>[11x]MSYHKENTPLTAGSQAASSSTASY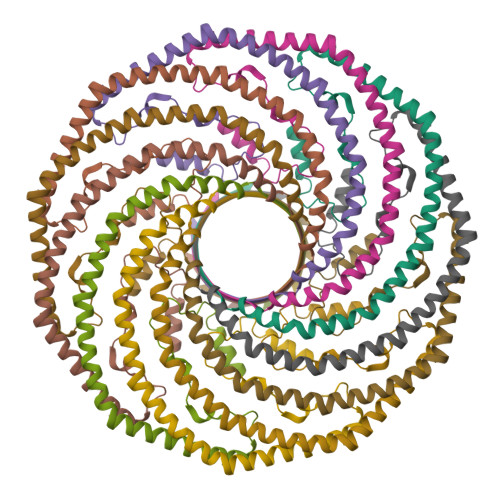QTPPYAPPSSVNHQQQQQARAAAPSYVGPTPTSTTTYPTIFTPGGFGAPPPSDPEAEEKYIERQLKYLGPISQVSDAYRLDTTTLKIEFDDSFPEVSKPGPALESVRKLNRILYEGMSDAIHIIFSLFLGFLAAITVGFFMGMARFMYTYMAGPFNQLMFLLIASLAPSWRAFFRAGMDPIFESGSLALSNIQVRLGMEGKARHKELKD Endoribonuclease YbeY is specific to the single-stranded RNA of ribosomal RNAs and small RNAs. This enzyme is essential for the maturation and quality control of ribosomal RNA in a wide range of bacteria and for virulence in some pathogenic bacteria. Early studies revealed that YbeY was involved in late-stage 70S ribosome quality control and the maturation of the 3' terminus of the 16S rRNA in bacteria. A later study revealed that Zn2+ is required for the nuclease activity of YbeY.

To gain structural information on YbeY from S. aureus (SaYbeY), we determined the crystal structure of full-length SaYbeY in complex with Zn2+ at a resolution of 1.9 Å. The SaYbeY structure consists of a four-stranded β-sheet and five α-helices. The active site cleft was identified between the protruding α5 and α2 from the flat surface of α3. The bound Zn2+ was found at the active site near α4, which was confirmed by the anomalous signal from the diffraction dataset collected at the Zn absorption edge wavelength. Two citrate molecules (Cit1 and Cit2) were assigned to the electron density maps based on the matched molecular shapes and crystallization solution containing 0.1 M sodium citrate (pH 5.5). Zn2+ is hexacoordinated by the three conserved histidine residues (His120, His124, and His130) of YbeY, α- and β-carboxylic groups and β-hydroxy group of the citrate molecule (Cit1). The binding of the Cit1 molecule is further stabilized by the ionic interaction with Arg58 from α-helix 2. The second citrate ion is bound by the carboxylic groups of the Asp65 side chain and the three histidine residues: His130 in the loop (α4-α5) and the two histidines in the hexahistidine tag. The hexahistidine tag was in the α-helical conformation and the loop conformation in the C-terminal end of SaYbeY, thus occupying the putative substrate-binding space between α3 and α5. In the modeled structure, the single-stranded RNA was located in the active site cleft between α2 and α5, and a phosphate backbone connecting nucleotides 3 and 4 was located near Zn2+ at the active site of SaYbeY.

> MAFTIDFSDHTGLVKDAWYKQIEDLLEFAKKEEHIEDDAELSVTFVDKQEIQEINRTYRDKDKVTDVISFALEEDEPEIDFSGLDIPRVLGDIIICTDVAQEQANNYGHSFERELGFLALHGFLHLLGYDHMTEADEKEMFGRQDTILNAYGLTRDHHHHHH> MDYKDDDDKPGLSCRFYQHKFPEVEDVVMVNVRSIAEMGAYVSLLEYNNIEGMILLSELSRRRIRSINKLIRIGRNECVVVIRVDKEKGYIDLSKRRVSPEEAIKCEDKFTKSKTVYSILRHVAEVLEYTKDEQLESLFQRTAWVFDDKYKRPGYGAYDAFKHAVSDPSILD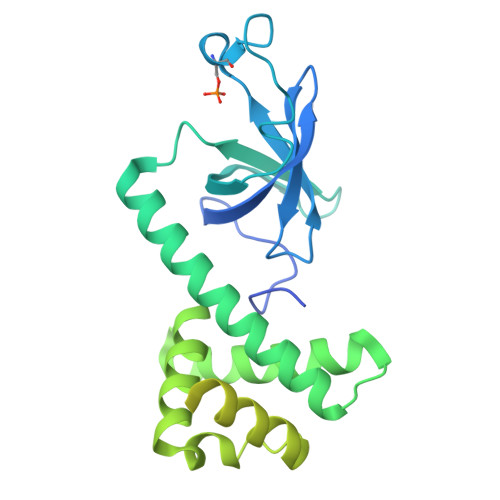SLDLNEDEREVLINNINRRLTPQAVKIRADIEVACYGYEGIDAVKEALRAGLNCSTENMPIKINLIAPPRYVMTTTTLERTEGLSVLSQAMAVIKEKIEEKRGVFNVQMEPKVVTDTDETELARQMERLERENAEVDGDDDAEEMEAKAED> QVAEDCMGLLQLLSNGTVLRSESIDLITQQIPFKNNQTVLFKDSIYHKPNNLHLRLYKPISASNRTALPVVVFFHGGGFCFGSRSWPHFHNFCLTLASSLNALVVSPDYRLAPEHRLPAAFEDAEAVLTWLWDQAVSDGVNHWFEDGTDVDFDRVFVVGDSSGGNIAHQLAVRFGSGSIELTPVRVRGYVLMGPFFGGEERTNSENGPSEALLSLDLLDKFWRLSLPNGATRDHHMANPFGPTSPTLESISLEPMLVIVGGSELLRDRAKEYAY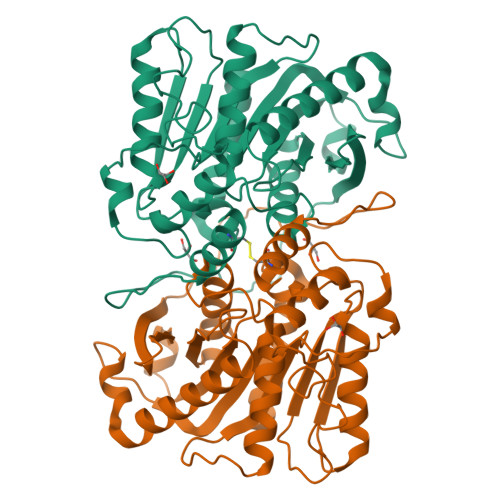KLKKMGGKRVDYIEFENKEHGFYSNYPSSEAAEQVLRIIGDFMNNLS> MMTMRGLLVGRMQPFHRGALQVIKSILEEVDELIICIGSAQLS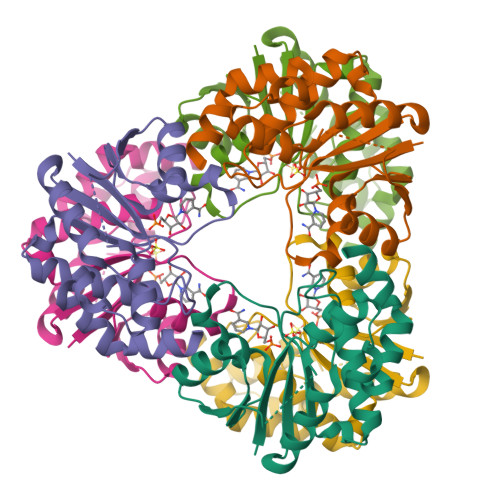HSIRDPFTAGERVMMLTKALSENGIPASRYYIIPVQDIECNALWVGHIKMLTPPFDRVYSGNPLVQRLFSEDGYEVTAPPLFYRDRYSGTEVRRRMLDDGDWRSLLPESVVEVIDEINGVERIKHLAKKEVSELGGIS> MIVLFVDFDYFYAQVEEVLNPSLKGKPV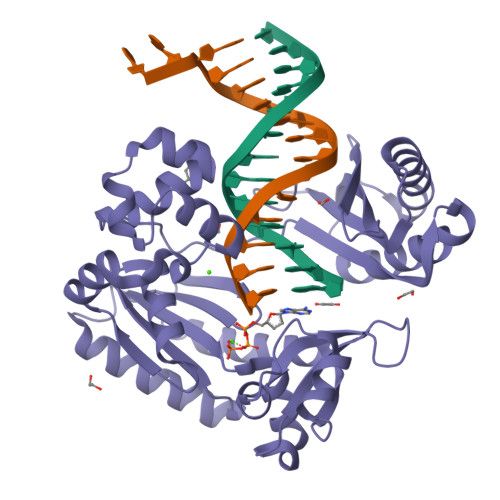VVCVFSGRFEDSGAVATANYEARKFGVKAGIPIVEAKKILPNAVYLPMRKEVYQQVSSRIMNLLREYSEKIEIASIDEAYLDISDKVRDYREAYNLGLEIKNKILEKEKITVTVGISKNKVFAKIAADMAKPNGIKVIDDEEVKRLIRELDIADVPGIGNITAEKLKKLGINKLVDTLSIEFDKLKGMIGEAKAKYLISLARDEYNEPIRTRVRKSIGRIVTMKRNSRNLEEIKPYLFRAIEESYYKLDKRIPKAIHVVAVTEDLDIVSRGRTFPHGISKETAYSESVKLLQKILEEDERKIRRIGVRFSKFIEAIGLDK> GAMAINLTSEKTLKEASTSMAPNVLKGNVIKNKAVASGKYVPFFGSSELSRFSAFHPSVLSEKYQRNYRPFLLGEAGTQSLTQAMVIHSMGDAIANKKAVFILSPQWFVKKGVPNDSFGAHYSQLQTYQWLANLTELTSGDQYLAQRLTKFPVVQKDKVLMETLANLQAGQLPQRSQRDYFIMNLRFLNREDELFSQIGMV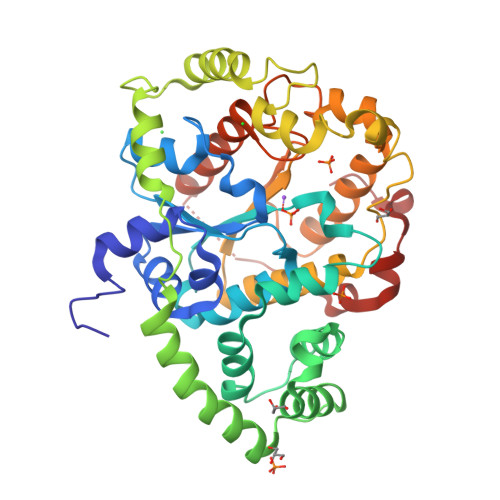SREPIVEKDMKQLPATYNFNELDQLAGKIAAKAINNNKFEISNGFYRQRIKPVLPKLAHSQKKWDYRFSPEYGDFQAALEQLAEKNVDVLFVIPPVNKRWSDYTGLSQDMLQQVARKLKYQLQEQGFTNIADFSTCSNERYFMADTIHLGWRGWLAVDRQVDEFMKQPASKKLAYQIDDRFYQTDWQQQNPLVLPQF> MAKIAYFKGLEQFILENSLIKNKPIKIVIGISMQSPHQISNEHKQSGDSFRAFVDLLRKTNEQCIRDENNNESAIRISELIVVITDGLHRHNLRLYKNVSTTEAESEAAGLGQKWVADNRQFLEAIGQCGISYKVIHWEELKSVAFNRYLQIVEEEYEKPNSEFRSIIDNLTQTHLEKL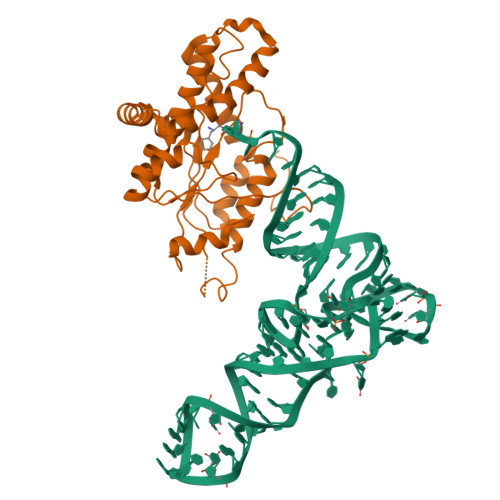VNFLLETRDSSFTQEDCVSATRKYLLEEAASAFEFASLKADGMTYPGPCSPGFKYIYDTYLSESNPLPFIEYGMRGGKKLPSFWKEESPVENALSGMPDEEFLIHHTSNFSNHHHHHH> SGPIDFWSSHPGQSSAAERELIGRFQDRFPTLSVKLIDAGKDYDEVAQKFNAALIGTDVPDVVLLDDRWWFHFALSGVLTALDDLFGQVGVDTTDYVDSLLADYEFNGRHYAVPYARSTPLFYYNKAAWQQAGLPDRGPQSWSEFDEWGPELQRVVGAGRSAHGWANADLISW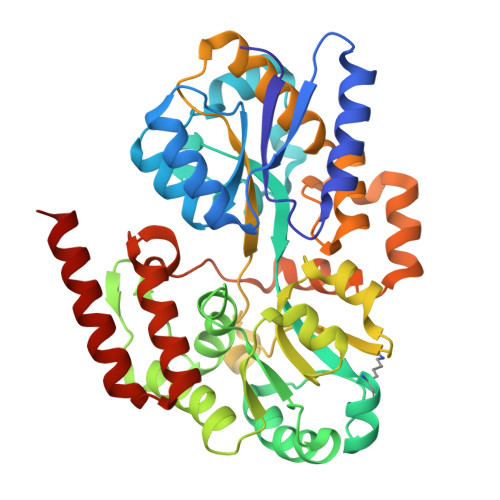TFQGPNWAFGGAYSDKWTLTLTEPATIAAGNFYRNSIHGKGYAAVANDIANEFATGILASAVASTGSLAGITASARFDFGAAPLPTGPDAAPACPTGGAGLAIPAKLSEERKVNALKFIAFVTNPTNTAYFSQQTGYLPVRKSAVDDASERHYLADNPRARVALDQLPHTRTQDYARVFLPGGDRIISAGLESIGLRGADVTKTFTNIQKRLQVILDRQIM> MEKEHNPYNSETNLETNLENTNIKSTGPSADDLKSRFKEGSIPLQTDYADLIDIADIGRRAVGKAPDQTNNPNSALELDDNSGLKIKINSTGGLKADQDGLSVKLKDKSLLADPNGLAVNAGRGVKINNDQLEVDGYHGIEIVNEGVKVKASNGINVNSDGVSVKAGNGISVSGKGVEVKAKDKGSISVDSDGIAVKYWDGGGIVATDNSGLYLKLEGGNTNNGWSGVSGLSLSKNGVKVKAGNGITVDSSGVSIDPKTVLPKGMIVMFSGSSAP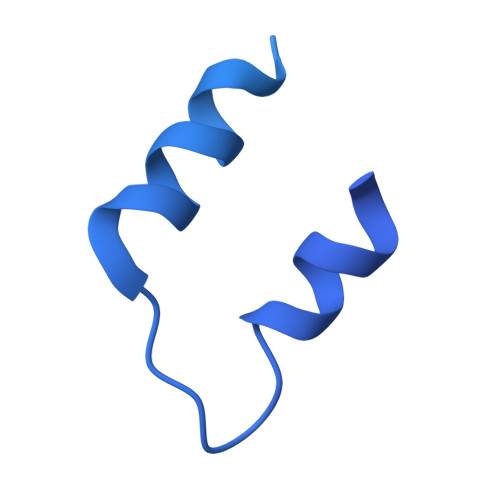TGWAFCDGNHGTPDLRSRFVMCSETISETGKSSNKASGSGNGKNYSRNTTSTTVSVSVTVKNTTLTESQIPYHYHIGGMGYWTNKGMKYGTEYYSEYASYIRNDLDSVMQSANGARYAYTSPSGGGQGHNHPATASSPSHDHSVNVIPPYYLLAFIMKL>[4x]AVKVGINGFGRIGRNVFRAALKNPDIEVVAVNDLTDANTLAHLLKYDSVHGRLDAEVSVNGNNLVVN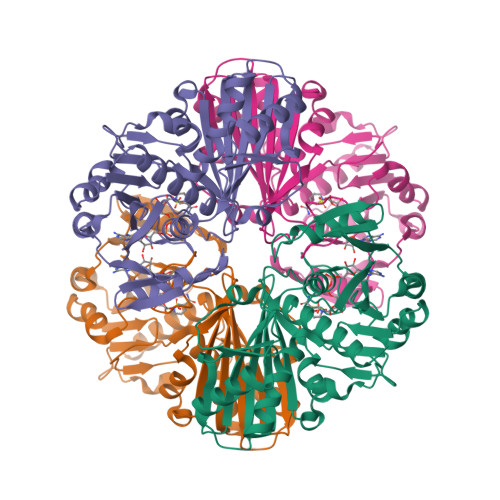GKEIIVKAERDPENLAWGEIGVDIVVESTGRFTKREDAAKHLEAGAKKVIISAPAKNEDITIVMGVNQDKYDPKAHHVISNASATTNCLAPFAKVLHEQFGIVRGMMTTVHSYTNDQRILDLPHKDLRRARAAAESIIPTTTGAAKAVALVLPELKGKLNGMAMRVPTPNVSVVDLVAELEKEVTVEEVNAALKAAAEGELKGILAYSEEPLVSRDYNGSTVSSTIDALSTMVIDGKMVKVVSWYDNETGYSHRVVDLAAYIASKGL> MHFEAYPPEVNSANIYAGPGPDSMLAAARAWRSLDVEMTAVQRSFNRTLLSLMDAWAGPVVMQLMEAAKPFVRWLTDLCVQLSEVERQIHEIVRAYEWAHHDMVPLAQIYNNRAERQILIDNNALGQFTAQIADLDQEYDDFWDEDGEVMRDYRLRVSD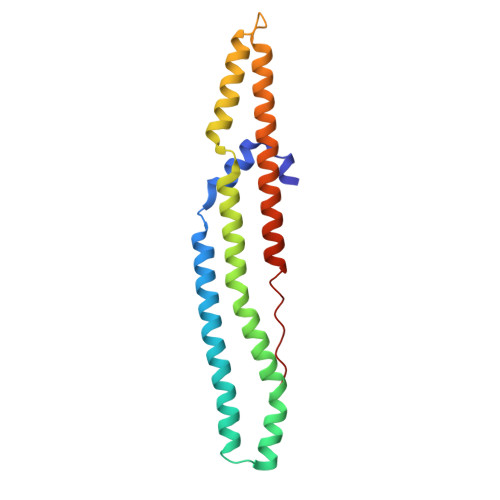ALSKLTPWKAPPPIA> MERYENLFAQLNDRREGAFVPFVTLGDPGIE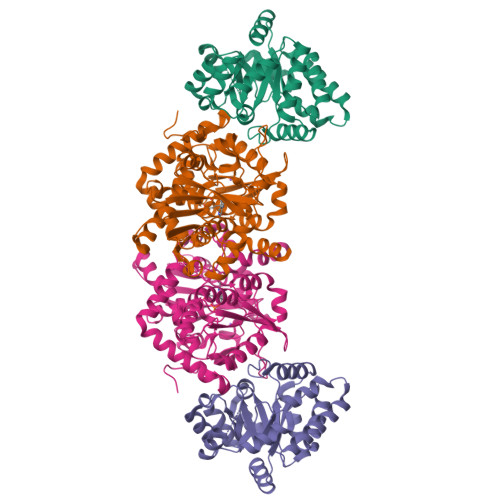QSLKIIDTLIDAGADALELGVPFSDPLADGPTIQNANLRAFAAGVTPAQCFEMLAIIREKHPTIPIGLLMYANLVFNNGIDAFYARCEQVGVDSVLVADVPVEESAPFRQAALRHNIAPIFICPPNADDDLLRQVASYGRGYTYLLSRSGVTGAENRGALPLHHLIEKLKEYHAAPALQGFGISSPEQVSAAVRAGAAGAISGSAIVKIIEKNLASPKQMLAELRSFVSAMKAASRA;> MTTLLNPYFGEFGGMYVPQILMPALNQLEEAFVSAQKDPEFQAQFADLLKNYAGRPTALTKCQNITAGTRTTLYLKREDLLHGGAHKTNQVLGQALLAKRMGKSEIIAEVGAGNHGVASALASALLGLKCRIYMGAKDVERQSPNVFRMRLMGAEVIPVHSGSATLKDACNEALRDWSGSYETAHYMLGTAAGPHPYPTIVREFQRMIGEETKAQILDKEGRLPDAVIACVGGGSNAIGMFADFINDTSVGLIGVEPGGHGIETGEHGAPLKHGRVGIYFGMKAPMMQTADGQIEESYSISAGLDFPSVGPQHAYLNSIGRADYVSITDDEALEAFKTLCRHEGIIPALESSHALAHALKMMREQPEKEQLLVVNLSGRGDKDIFTVHDILKARGEI> DGLNGTMMQYYEWHLENDGQHWNRLHDDAAALSDAGITAIWIPPAYKGNSQADVGYGAYDLYDLGEFNQKGTVRTKYGTKAQLERAIG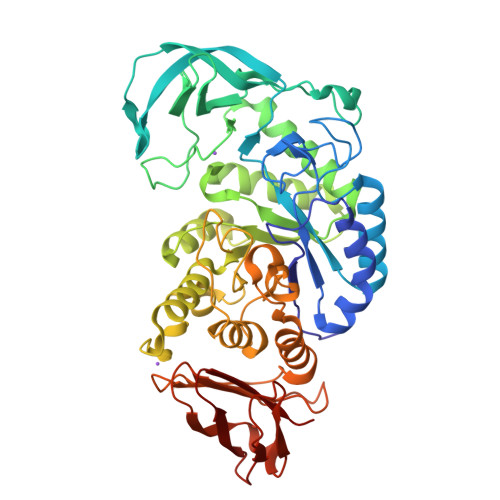SLKSNDINVYGDVVMNHKMGADFTEAVQAVQVNPTNRWQDISGAYTIDAWTGFDFSGRNNAYSDFKWRWFHFNGVDWDQRYQENHIFRFANTNWNWRVDEENGNYDYLLGSNIDFSHPEVQDELKDWGSWFTDELDLDGYRLDAIKHIPFWYTSDWVRHQRNEADQDLFVVGEYWKDDVGALEFYLDEMNWEMSLFDVPLHYNFYRASQQGGSYDMRNILRGSLVEAHPMHAVTFVDNHDTQPGESLESWVADWFKPLAYATILTREGGYPNVFYGDYYGIPNDNISAKKDMIDELLDARQNYAYGTQHDYFDHWDVVGWTREGSSSRPNSGLATIMSNGPGGSKWMYVGRQNAGQTWTDLTGNNGASVTINGDGWGEFFTNGGSVSVYVNQ>MARKKNYRPLIALAALAVAALAMATLTFTNLTYWLINATLPPAMKYPGTDTTITRSDSSGYNRYVYVSYYYDPSTGYNVTRISIVGFTGDPTNYTNVLQLCNKYYSGTLYAKLVAVGTVGTTNYESYIKDFRVYFVNPTTTPNYVQFQGTSV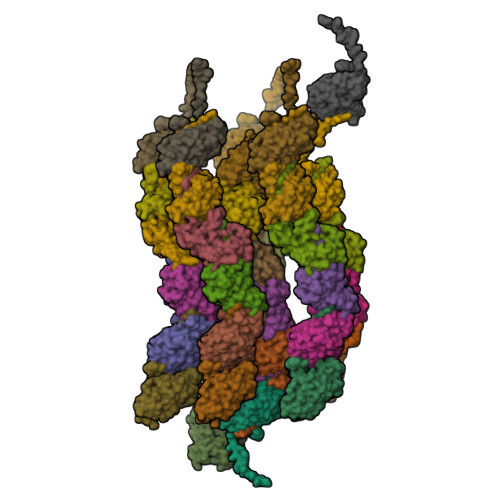TQSATGSVSIGPGQCATVGAYVLVDPSLPTSARDGKTVIATYQVNVVFSTSP[6x]> SAGATAADGPCALRELSVDLRAERSVLIPETYQANNCQGVCGWPQSDRNPRYGNHVVLLLKMQARGAALARPPCCVPTAYAGKLLISLSEERISAHHVP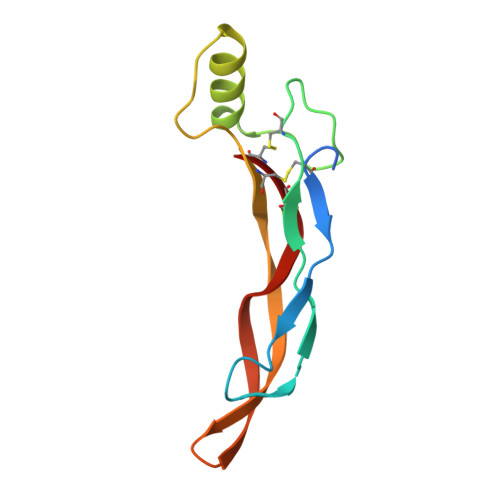NMVATECGCR4-(4-{1-[(6-aminopyridin-2-yl)methyl]-5-(2-chlorophenyl)-1H-pyrrol-2-yl}phenoxy)butanenitrile 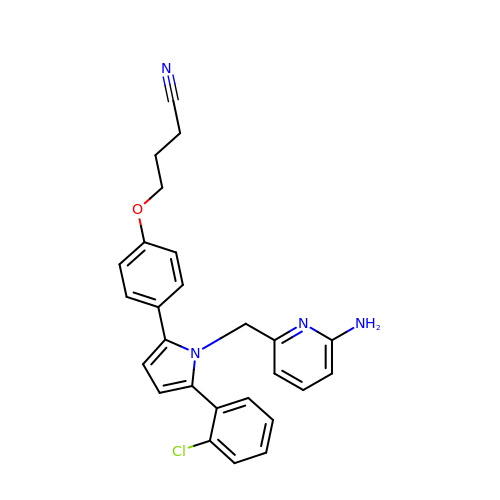| C26 H23 Cl N4 O | CERJQPWNRISSQS-UHFFFAOYSA-N2-(benzimidazol-1-yl)-~{N}-(2-phenylethyl)ethanamide | C17 H17 N3 O | 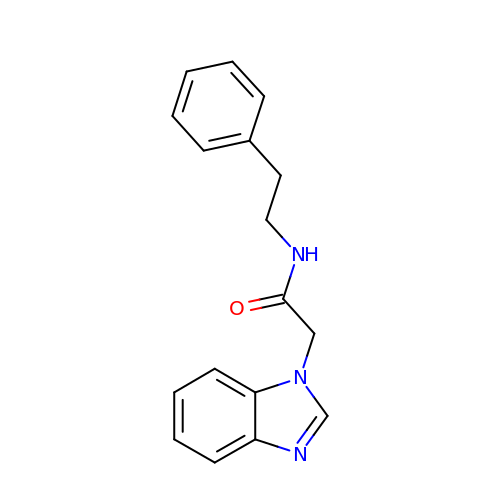CAHHWKPTYNNMOV-UHFFFAOYSA-N CD23, also designated FcϵRII and CLEC4J, is a cell-surface receptor for the Fc domain of IgE, which regulates IgE synthesis. The extracellular portion of CD23 consists of a C-terminal C-type lectin-like domain attached to the membrane by an extended neck region. The results reported here demonstrate that CD23 from both cows and mice does bind to sugars in a Ca2+-dependent manner but that this activity has been lost in most primate species, including humans. The structure of cow CD23 confirms the presence of the four disulfide bonds predicted from the alignment with other C-type CRDs and also shows that there are two bound Ca2+, representing the conserved Ca2+ found at sugar-binding sites in C-type CRDs and the adjacent accessory site.

The mechanism of sugar binding to cow CD23 was examined by X-ray crystallography. Crystals of the CRD from cow CD23 were obtained under conditions that allow binding of sugar ligands: in the presence of 5 mm Ca2+. The cow CD23 structure shows a typical C-type CRD fold, and the bound sugar ligands are well-defined. In the secondary binding site, Ser277, which forms a hydrogen bond with O6 of GlcNAc, is found in cow and mouse, but not human, CD23, and Met263, which contacts C4 of GlcNAc, is conserved in cow, mouse, and human CD23. However, Leu265 in cow CD23, which contacts the carbonyl oxygen on the GlcNAc acetamido group, is replaced by Arg in mouse and human CD23, and it is not clear whether an equivalent contact would be made. The surface near the primary binding site lacks obvious protrusions, so it is hard to define a secondary or extended binding site that would favor particular oligosaccharide ligands or occlude others. The relatively open binding site allows interaction with these monosaccharides in multiple contexts, although some types of oligosaccharide ligands appear to be favored as a result of a small number of interactions with sugars beyond the terminal residues.

> ANGSVCNTCPEAWIYFQKKCYYFGEGAKKWIQARYACENLHGRLVSIHSPEEQDFLTKRANWRGSWIGLRDLDIEGEFIWMDNQPLDYSNWQPGEPNDAGQGENCVMMLGSGKWNDAFCGSELHGWVCDRLATC>[4x]SLVQLWKMI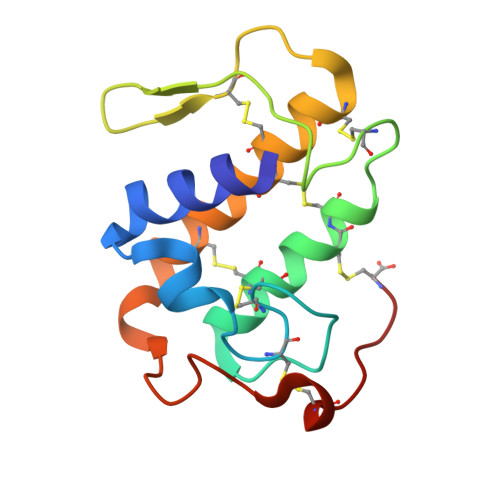FQETGKEAAKNYGLYGCNCGVGRRGKPKDATDSCCYVHKCCYKKVTGCNPKMDSYSYSWKNKAIVCGEKNPPCLKQVCECDKAVAICLRENLGTYNKKYTIYPKPFCKKADTC>SNAMDMVTVTAKTVEEAVTKALIELQTTSDKLTYEIVEKGSAGFLGIGSKPAIIRAKRKETLQDKAIEFLEQVFDAMNMAVDISVEYNETEKEMNVNLKGDDMGILIGKRGQTLDSLQYLVSLVVNKSSSDYIRVKLDTENYRERRKETLETLAKNIAYKVKRTKRSVSLEPMNPYERRIIHA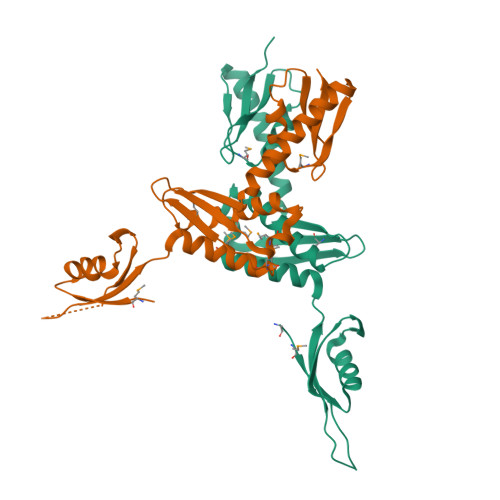ALQNDKYVVTRSDGEEPFRHVIISLKRENRRDRNDRSDRNEK[3x]> MCIEFAFKKAGIPIVRNFLHSTEGVIYGLPQRVQ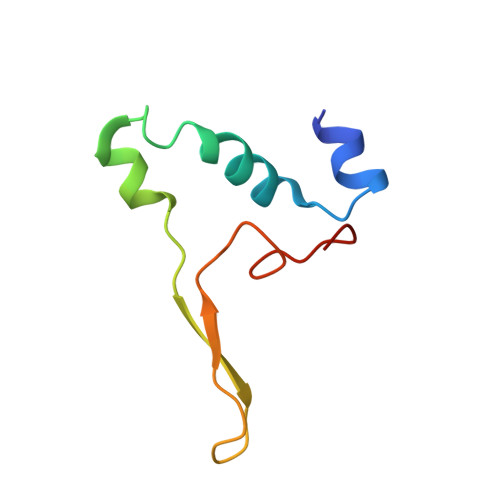RNLAINYTVKQYKEGKAVSAKTIKTLQEAFPSKGDTK> IETVPVKLKPGMDGPKVKQWPLTEEKIKALVEICTEMEKEGKISKIGPENPYNTPVFAIKKKDSTKWRKLVDFRELNKRTQDFWEVQLGIPHP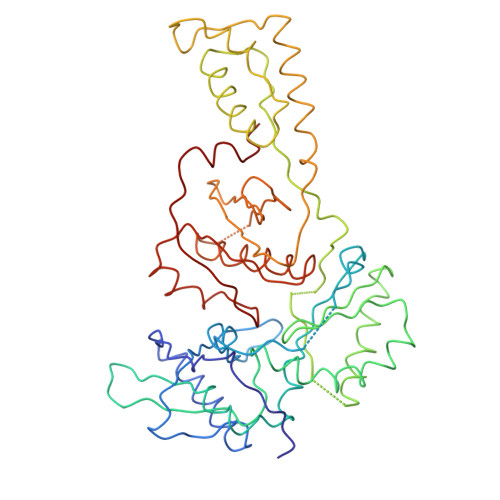AGLKKKKSVTVLDVGDAYFSVPLDEDFRKYTAFTIPSINNETPGIRYQYNVLPQGWKGSPAIFQSSMTKILEPFRKQNPDIVIYQYMDDLYVGSDLEIGQHRTKIEELRQHLLRWGLTTPDKKHQKEPPFLWMGYELHPDKWTVQPIVLPEKDSWTVNDIQKLVGKLNWASQIYPGIKVRQLCKLLRGTKALTEVIPLTEEAELELAENREILKEPVHGVYYDPSKDLIAEIQKQGQGQWTYQIYQEPFKNLKTGKYARMRGAHTNDVKQLTEAVQKITTESIVIWGKTPKFKLPIQKETWETWWTEYWQATWIPEWEFVNTPPLVKLWYQLEK> PISPIETVPVKLKPGMDGPKVKQWPLTEEKIKALVEICTEMEKEGKISKIGPENPYNTPVFAIKKKDSTKWRKLVDFRELNKRTQDFWEVQLGIPHPAGLKKKKSVTVLDVGDAYFSVPLDEDFRKYTAFTIPSINNETPGIRYQYNVLPQGWKGSPAIFQSSMTKILEPFKKQNPDIVIYQYMDDLYVGSDLEIGQHRTKIEELRQHLLRWGLTTPDKKHQKEPPFLWMGYELHPDKWTVQPIVLPEKDSWTVNDIQKLVGKLNWASQIYPGIKVRQLSKLLRGTKALTEVIPLTEEAELELAENREILKEPVHGVYYDPSKDLIAEIQKQGQGQWTYQIYQEPFKNLKTGKYARMRGAHTNDVKQLTEAVQKITTESIVIWGKTPKFKLPIQKETWETWWTEYWQATWIPEWEFVNTPPLVKLWYQLEKEPIVGAETFYVDGAANRETKLGKAGYVTNKGRQKVVPLTNTTNQKTELQAIYLALQDSGLEVNIVTDSQYALGIIQAQPDKSESELVNQIIEQLIKKEKVYLAWVPAHKGIGGNEQVDKLV;> PISPIETVPVKLKPGMDGPKVKQWPLTEEKIKALVEICTEMEKEGKISKIGPENPYNTPVFAIKKKDSTKWRKLVDFRELNKRTQDFWEVQLGIPHPAGLKKKKSVTVLDVGDAYFSVPLDEDFRKYTAFTIPSINNETPGIRYQYNVLPQGWKGSPAIFQSSMTKILEPFKKQNPDIVIYQYMDDLYVGSDLEIGQHRTKIEELRQHLLRWGLTTPDKKHQKEPPFLWMGYELHPDKWTVQPIVLPEKDSWTVNDIQKLVGKLNWASQIYPGIKVRQLSKLLRGTKALTEVIPLTEEAELELAENREILKEPVHGVYYDPSKDLIAEIQKQGQGQWTYQIYQEPFKNLKTGKYARMRGAHT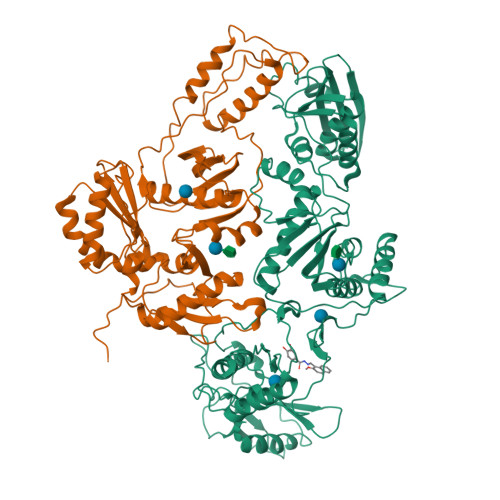NDVKQLTEAVQKITTESIVIWGKTPKFKLPIQKETWETWWTEYWQATWIPEWEFVNTPPLVKLWYQL Two key enzymes, i.e., 6-phosphogluconolactonase (Pgl) and 6-phosphogluconate dehydrogenase (Gnd or 6PGDH), from oxPPP were identified as Ag+-binding proteins by LC-GE-ICP-MS. As the third enzyme in oxPPP, 6PGDH converts 6-phosphogluconate (6PG) to ribulose 5-phosphate (Ru5P) with the concomitant reduction of NADP+ to NADPH. Since oxPPP is the major NAPDH-generating pathway in S. aureus, we therefore further measured the NADPH/NADP+ ratio in S. aureus exposed to Ag+. With the recombinant 6PGDH, we show that Ag+ binds to 6PGDH and inhibits its activity in a non-competitive manner.

Attempts on direct crystallization of Ag-bound 6PGDH were not successful. Thus, we crystallized apo-6PGDH, which stands for the first crystal structure of 6PGDH from S. aureus, and then soaked the crystals into cryo-protectants containing 0.5 mM Ag+ for 2 h, allowing the protein to bind Ag+ in its packed form.

>MTQQIGVIGLAVMGKNLAWNIESRGYSVSVFNRSSEKTDLMVEESKGKNIHPTYSLEEFVNSLEKPRKILLMVQAGKATDATIDSLLPLLDDGDILIDGGNTNYQDTIRRNKALAQSAINFIGMGVSGGEIGALTGPSLMPGGQEEAYNKVADILDAIAAKAKDGASCVTYIGPNGAGHYVKMVHNGIEYADMQLIAESYAMMKELLGMSHEDIAQTFKDWNAGELESYLIEITGDIFMKLDENKEALVEKILDTAGQKGTGKWTSINALELGIPLTIITESVFARFISSIKEERVNASKELNGPKASFDGDKKDFLEKIRKALYMSKICSYAQGFAQMRKASEDNEWNLKLGDLAMIWREGCIIRAQFLQKIKDAYDNNPGLQNLLLDPYFKNIVTEYQDALRDVVATGVQNGVPTPGFSSSINYYDSYRAADLPANLIQAQRDYFGAHTYERKDKEGVFHTQWIEE[4x]> GSKNYIEMKPHPWFFGKIPRAKAEEMLSKQRHDGAFLIRESE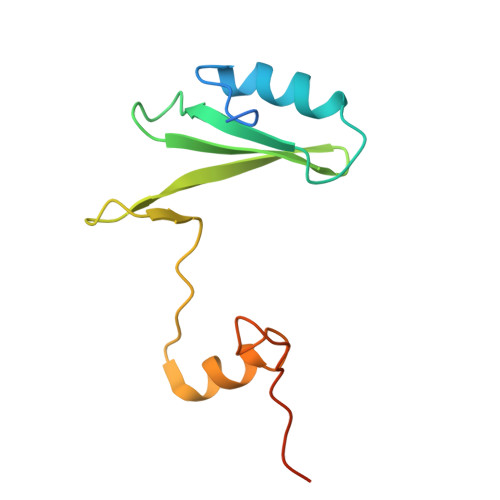SAPGDFSLSVKFGNDVQHFKVLRDGAGKYFLWVVKFNSLNELVDYHRSTSVSRNQQIFLRDIEQVPQQPTYV> QQSCNTPSNRACWTDGYDINTDYEVDSPDTGVVRPYTLTLTEVDNWTGPDGVVKEKVMLVNNSIIGPTIFADWGDTIQVTVINNLETNGTSIHWHGLHQKGTNLHDGANGITECPIPPKGGRKVYRFKAQQYGTSWYHSHFSAQYGNGVVGAIQINGPASLPYDTDLGVFPISDYYYSSADELVELTKNSGAPFSDNVLFNGTAKHPETGEGEYANVTLTPGRRHRLRLINTSVENHFQVSLVNHTMTIIAADMVPVNAMTVDSLFLGVGQRYDVVIEASRTPGNYWFNVTFGGGLLCGGSRNPYPAAIFHYAGAPGGPPTDEGKAPVDHNCLDLPNLKPVVARDVPLSGFAKRPDNTLDVTLDTTGTPLFVWKVNGSAINIDWGRPVVDYVLTQNTSFPPGYNIVEVNGADQWSYWLIENDPGAPFTLPHPMHLHG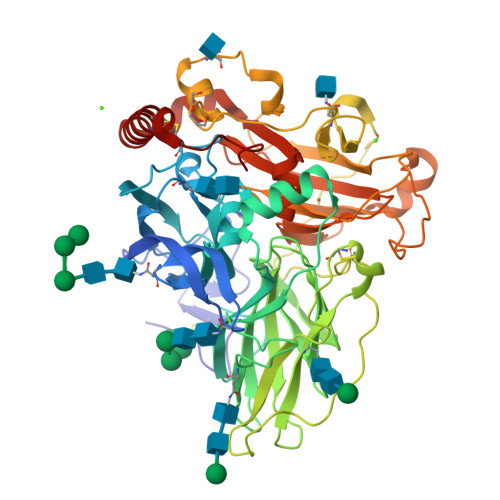HDFYVLGRSPDESPASNERHVFDPARDAGLLSGANPVRRDVTMLPAFGWVVLAFRADNPGAWLFHCHIAWHVSGGLGVVYLERADDLRGAVSDADADDLDRLCADWRRYWPTNPYPKSDSGL> ALANTFLVKEDSKNVTAYTPFATPITDSKSDLVSLAQLDSSYQIADQTIHNTNLFVLFKSRDVKVKYESSGSNNISFDSTSQGEKPSYVVEFTNSTNIGIKWTMVKKYQLDVPNVSSDMNQVLKNLILEQPLTKYTLNSSLAKEKGKTQREVHLGSGQANQWTSQRNQHDLNNNPSPNASTGFKLTTGNAYRKLSESWPIYEPIDGTKQGKGKDSSGWSSTEENEAKNDAPSVSGGGSSSGTFNKYLNTKQALESIGILFDDQTPRNVITQLYYASTSKLAVTNNHIVVMGNSFLPSMWYWVVERSAQENASNKPTWFANTNLDWGEDKQKQFVENQLGYKETTSTNSHNFHSKSFTQPAYLISGIDSVNDQIIFSGFKAGSVGYDSSSSSSSSSSSSTKDQALAWSTTTSLDSKTGYKDLVTNDTGLNGPINGSFSIQDTFSFVVPYSGNHTNNGTTGPIKTAYPVKKDQKSTVKINSLINATPLNSYGDEGIGVFDALGLNYNFKSNQERLPSRTDQIFVYGIVSPNELRSAKSSADSTGSDTKVNWSNTQ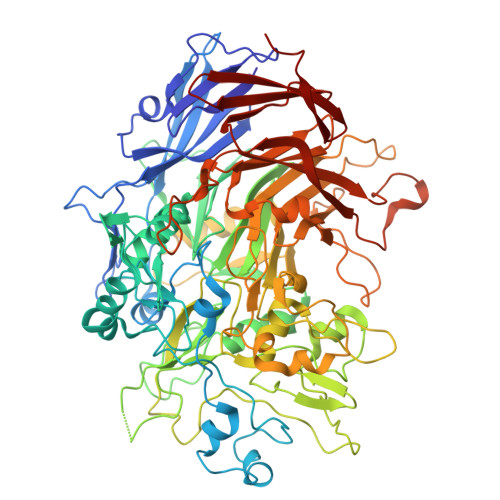SRYLPVPYNYSEGIIDADGFKRPENRGASVTTFSGLKSIAPDGFANSIANFSVGLKAGIDPNPVMSGKKANYGAVVLTRGGVVRLNFNPGNDSLLSTTDNNIAPISFSFTPFTAAESAVDLTTFKEVTYNQESGLWSYIFDSSLKPSHDGKQTPVTDNMGFSVITVSRTGIELNQDQATTTLDVAPSALAVQSGIQSTTQTLTGVLPLSEEFSAVIAKDSDQNKIDIYKNNNGLFEIDTQLSNHHHHHH>[4x]GPGSMNVAISPGVTAGNSLPFVLFGGINVLESLDFTLDVCGEYVAVTRKLGIPFVFKASFDKANRSSIHSYRGVGLDEGLKIFAEVKARFGVPVITDVHEAEQAAPVAEIADVLQVPAFLARQTDLVVAIAKAGKPVNVKKPQFMSPTQLKHVVSKCGEVGNDRVMLCERGSSFGYDNLVVDMLGFRQMAETTGGCPVI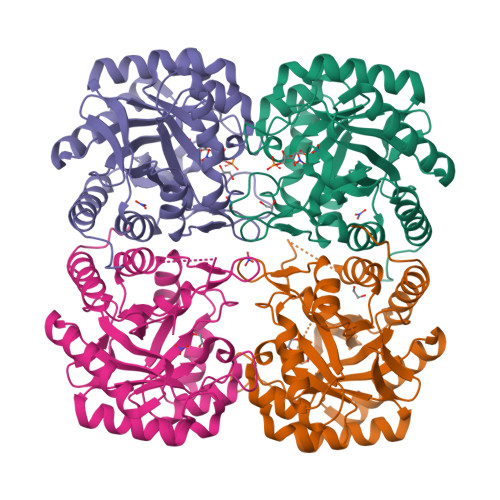FDVTHSLQCRDPLGDASGGRRRQVLDLARAGIAVGIAGLFLEAHPDPDRARCDGPSALPLHQLEGLLSQMKAIDDLVKRMPALEIR>MSTLANLTEVLFRLDFDPDTAVYHYRGQTLSRLQCRTYILSQASQLARLLKPGDRVVLALNDSPSLACLFLACIAVGAIPAVINPKSREQALADIAADCQASLVVREADAPSLSGPLAPLTLRAAAGRPLLDDFSLDALVGPADLDWSAFHRQDPAAACFLQYTSGSTGAPKGVMHSLRNTLGFCRAFATELLALQAGDRLYSIPKMFFGYGMGNSLFFPWFSGASALLDDTWPSPERVLENLVAFRPRVLFGVPAIYASLRPQARELLSSVRLAFSAGSPLPRGEFEFWAAHGLEICDGIGATEVGHVFLANRPGQARADSTGLPLPGYECRLVDREGHTIEEAGRQGVLL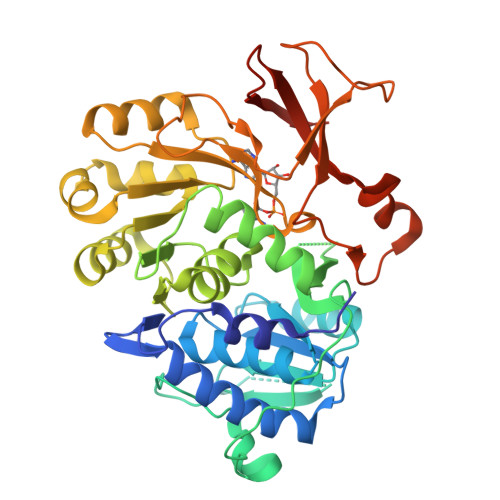VRGPGLSPGYWRASEEQQARFAGGWYRTGDLFERDESGAYRHCGREDLEHHHHHH[2x]> MPVPNPTMPVKGAGTTLWVYKGSGDPYANPLSDVDWSRLAKVKDLTPGELTAESYDDSYLDDEDADWTATGQGQKSAGDTSFTLAWMPGEQGQQALLAWFNEGDTRAYKIRFPNGTVDVFRGWVSSIGKAVTAK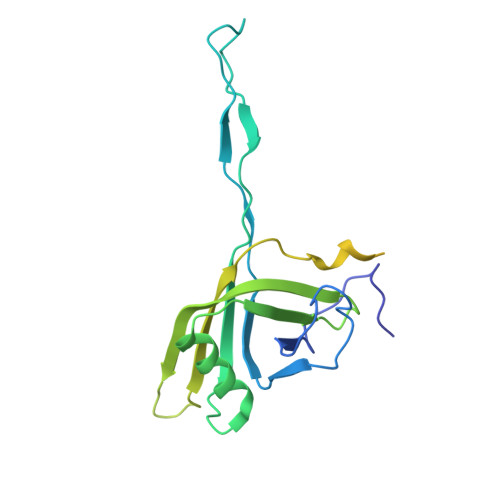EVITRTVKVTNVGRPSMAEDRSTVTAATGMTVTPASTSVVKGQSTTLTVAFQPEGVTDKSFRAVSADKTKATVSVSGMTITVNGVAAGKVNIPVVSGNGEFAAVAEITVTAS3-METHYL-BETA-D-ASPARTIC 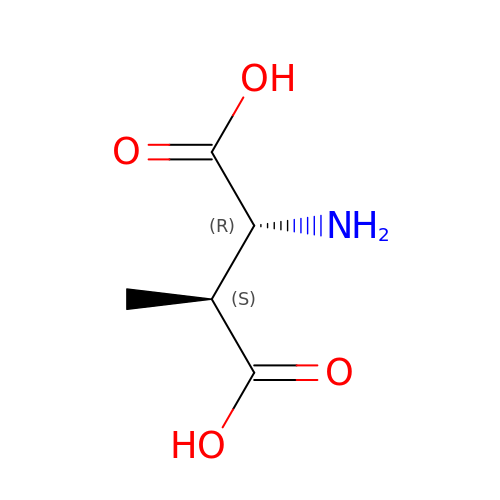ACID | C5 H9 N O4 | LXRUAYBIUSUULX-STHAYSLISA-N> MKNIKKNQVMNLGPNSKLLKEYKSQLIELNIEQFEAGIGLILGDAYIRSRDEGKTYCMQFEWKNKAYMDHVCLLYDQWVLSPPHKKERVNHLGNLVITWGAQTFKHQAFNKLANLFIVNNKKTIPNNLVENYLTPMSLAYWFMDDGGKWDYNKNSTNKSIVLNTQSFTFEEVEYLVKGLRNKFQLNCYVKINKNKPIIYIDSMSYLIFYNLIKPYLIPQMMYKLPNTISSETFLK;> MKNIKKNQVMNLGPNSKLLKEYKSQLIELNIEQFEAGIGLILGDAYIRSRDEGKTYCMQFEWKNKAYMDHVCLLYDQWVLSPPHKKERVNHLGNLVITWGAQTFKHQAFNKLANLFIVNNKKTIPNNLVENYLTPMSLAYWFMDDGGKWDYNKNSTNTSIVLNTQSFTFEEVEYLVKGLRNKFQLNCYVKINKNKPIIYIDSMSYL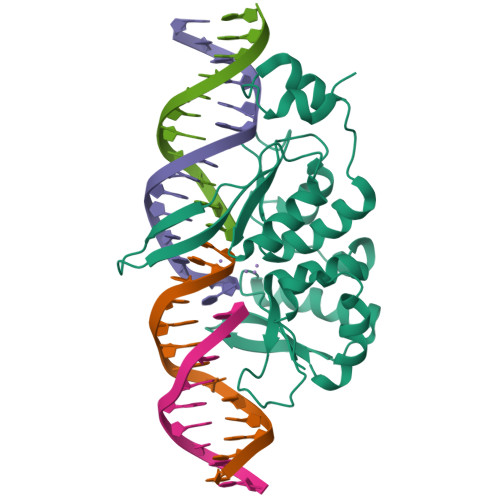IFYNLIKPYLIPQMMYKLPNTISSETFLK> KGGAXRHRKI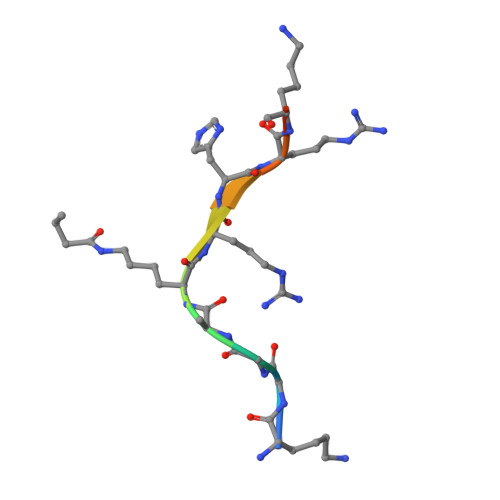L>[2x]MRPENVVVKKPKKLRDYQQTAKENALAHFKENDRGQLIMAPGTGKTFTSLKISEALSKDKNGPFKVLYLVPSIQLLTQTLRGWNNDTELTITSMAVTSDRDASRGTDGTEDIKASDIGYPATTSSKKILQNWHDFESLPKQTDMLVVFSTYQSIEVIGEAQKEGFPEFDFIISDEAHRTTGAHEAAKEASAFSKVHSNNNVKGLKRMYQTATPKIYGESAKKNAKDKSILLSSMDDESKYGEVFFRMGFGQAVSRDILTDYKVMVLAVDEAAIQKDMQRTLADPENGLNIDDVGRIVGIWNGMMRRNGYKNPIKNSPYDGAPLERAIAFTRTIEESKKVSSQFEEVVNEYISEAIEDESIHLSMRHADGKMNALQKGEILDWLADPNKPADEARIVSNVRFLTEGIDIPTLDAVIFLSPKKSQVDIVQAVGRIMRKAEGKDYGYIILPIVIPTGEKPETILDNNKNYETVWQVINALRSVDERFEAMIDKLNMAKPKQLKVIGVGSAPEQVNDQDKTIENTPVQTELELEWNKFEGAIFGKIVQKVGDRKYLENWSKDVAKIAERQINWIKNKLSDKKDPISLEFKKFVSSLQHNINDSIDEKQAAEMLSQHLITKPIFEALFSEYSFVNQNPVSQAMESIVSELEKAGFAKEQENLEPLYESVRMRAEGIEKAEDKQKIIVTLYDKFFKTAFKATTERLGIVFTPIEVVDFIVHSVDDVLKKHFGKSLASKDVHILDPFTGTGTFIVRTLTYLKEQMDAGEISLSDITRKFMKELHANEIVLLSYYIAAINIEATFDEINGEEEGYVPFEGIVLTDTFESTETEETLDDDYFGTNDERLKRQQEVPITAIIGNPPYSKGQSNENDNNKNIEYPRLFKSIADSYVKNSKTTSVLGMYDSYVLSIRWASNRLNDKGVIGFVSNGSYIDSQSADGLRKSLFKEFNHLYIFNLRGDQRTQGETSRKEGGKIFGSGSRT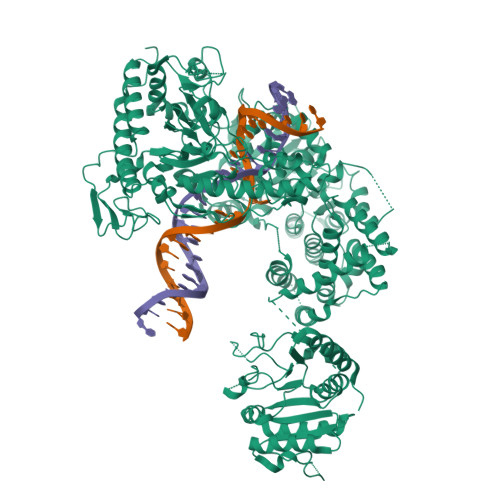SIAISILVKDDSDNHEVHYHDIGDYLTRDDKLDILRDKESILNIDWENISPDENNDWINQRDQNYLNYRPLADENGSIFSVKDIGIVTNRDAWVSNFSKINVSDNVQIMIKNYNLEVDRLENIDVKLNDKTVVDYVTNDERKISWSRSLKQRAARREKTQFSHSDIMLAMYRPFTKKYLYRNRFLNENVRKTYQTFPDKNSKNLLINISGQGDKADFATLISEYLSDMHVIGGQARNLPRFTYETDGMFAGRTDNIVSDDEFYYVYGVLHSSAYRKRYANDLKKDLPRIPLLKNKDKYVEIGRKLSDLHLNYENQPIWDGIEVEISQPDYRVKKMKHPKKGVLDTIIYNESITIKNIPERAYEYVVNGRPAIEWIIDQYQVKTDKKSGITDDPNEFSDNPKYILNLLLSVITVSMRTLELIEELPEFEIQE>GSAKDPMAIVVKVVNGKIQEFENGIHKRTYGSNIVAADTDGHIVAAVTAKGKVEEFENGIHKRTYGSNAINVQVSGGVVAVTTS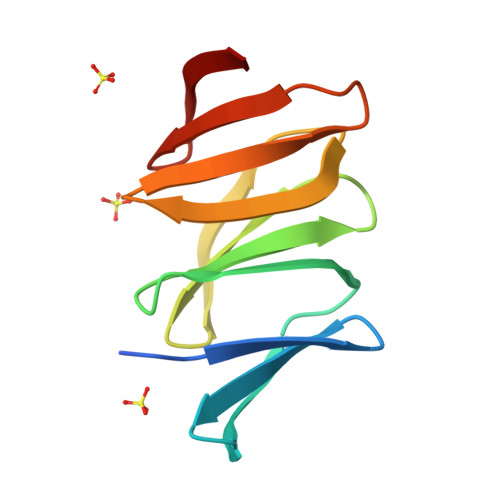KGKVEEYKNGIHKRTY[4x]>GGVEVLEVKTGVDAITEVECFLNPEMGDPDENLRGFSLKLSVQNDFSSDSPQRKMLPCYSTARIPLPNLNEDLTSGNLLMWEAVTVQTEVIGITSMLNLHAGSQKVHEHGGGKPIQGSNFHFFAVGGEPLEMQ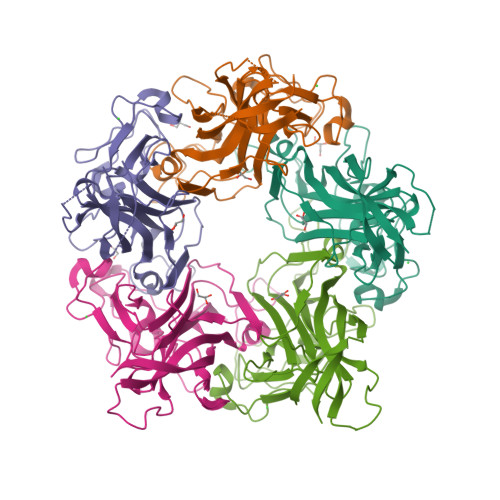GVLMNYRSKYPDGTITPKNPTAQSQVMNTDHKAYLDKNNAYPVECWVPDPSRNENARYFGTFTGGENVPPVLHVTNTATTVLLDEQGVGPLCKADSLYVSAADICGLFTNSSGTQQWRGLARYFKIRLRKRSVKNPYP[5x]> MDDEEIEKGVTSIVAEVTELDEKEIWEKRDANFFQDLEIDSLLALEILALIEKKFKVQIPEEKLVDITSLSATIGLTKSVLAESGKLEHHHH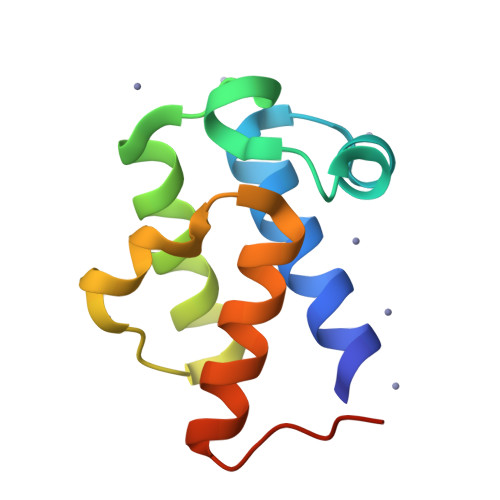HH>[2x]ANE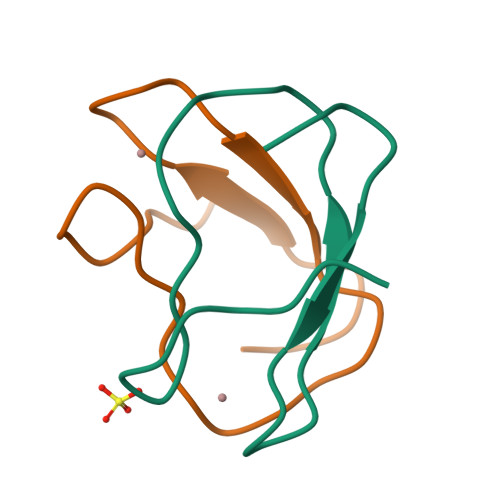GDVYKCELCGQVVKVLEEGGGTLVCCGEDMVKQ>GPMATESPNSVQKIVVHLRATGGAPILKQSKFKVSGSDKFANVIDFLRRQLHSDSLFVYVNSAFSPNPDESVIDLYNNFGFDGKLVVNYACSMAWG[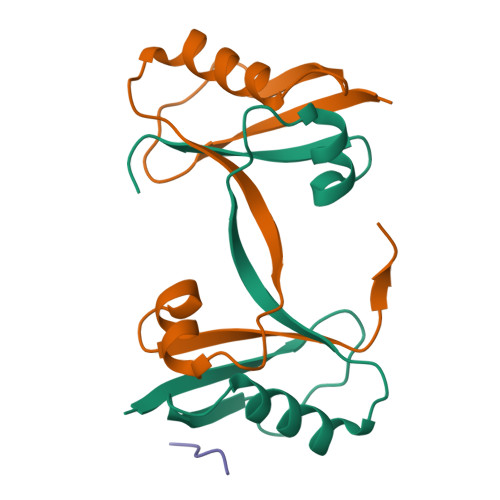14x];>[4x]DDIPDMEEFDE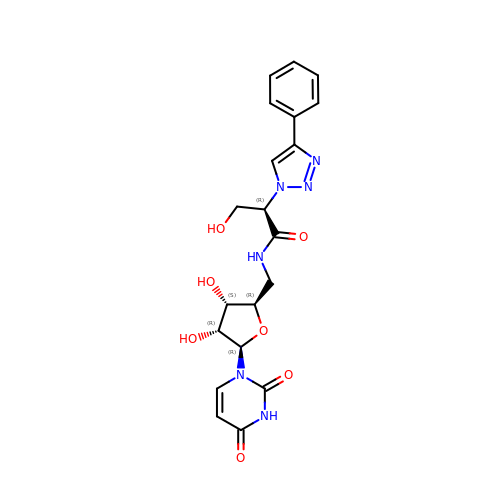5'-deoxy-5'-{[(2R)-3-hydroxy-2-(4-phenyl-1H-1,2,3-triazol-1-yl)propanoyl]amino}uridine | C20 H22 N6 O7 | FHKBVNPNDGIXHL-RKVZRBGQSA-N>PIELLPETPSQTAGPYVHIGLALEAAGNPTRDQEIWNRLAKPDAPGEHILLLGQVYDGNGHLVRDSFLEVWQADANGEYQDAYNLENAFNSFGRTATTFDAGEWTLHTVKPGVVNNAAGVPMAPHINISLFARGINIHLHTRLYFDDEAQANAKCPVLNLIEQPQRRETLIAKRCEVDGKTAYRFDIRIQGEGETVFFDF[6x];>PAQDNSRFVIRDRNWHPKALTPDYKTSIARSPRQALVSIPQSISETTGPNFSHLGFGAHDHDLLLNFNNGGLPIGERIIVAGRVVDQYGKPVPNTLVEMWQANAGGRHRHKNDRYLAPLDPNFGGVGRCLTDSDGYYSFRTIKPGPYPWRNGPNDWRPAHIHFGISGPSIATKLITQLYFEGDPLIPMCPIVKSI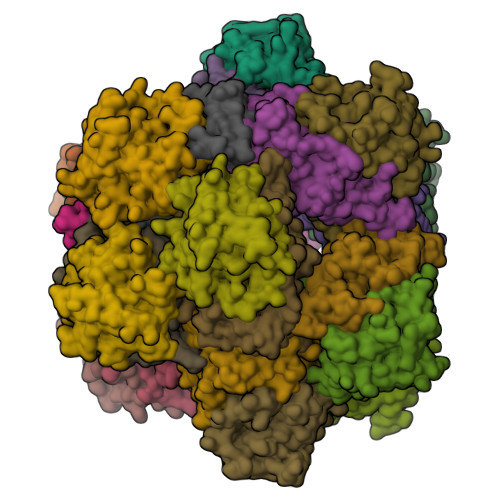ANPEAVQQLIAKLDMNNANPMDCLAYRFDIVLRGQRKTHFENC[6x]> MYLGRILAVGRNSNGSFVAYRVSSRSFPNRTTSIQEERVAVVPVEGHERDVFRNPYIAYNCIRIVGDTAVVSNGSHTDTIADKVALGMNLRDAIGLSLLAMDYEKDEL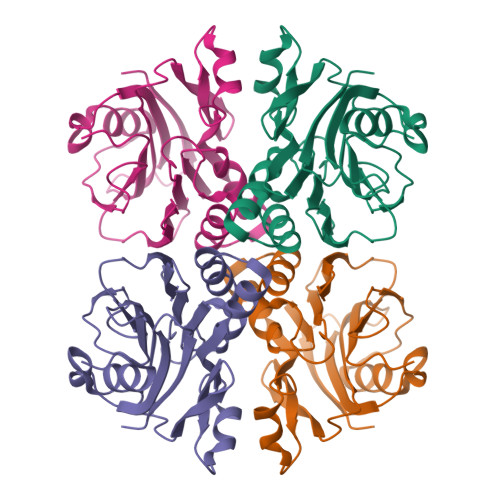NTPRIAAAINGSEAFIGIVTADGLMVSRVPEETPVYISTYEQTEPAATEFKAGSPEEAAEFILKGGEFAAFTHPVTAAAAFNDGEGWNLATREM> GLIVDTRDVEERVHVMRETKLAPTVAHGVFNPEFGPAALSNKDPRLNEGVVLDEVIFSKHKGDTKMSAEDKALFRRCAADYASRLHSVLGTANAPLSIYEAIKGVDGLDAMEPDTAPGLPWALQGKRRGALIDFENGTVGPEVEAALKLMEKREYKFACQTFLKDEIRPMEKVRAGKTRIVDVLPVEHILYTRMMIGRFCAQMHSNNGPQIGSAVGCNPDVDWQRFGTHFAQYRNVWDVDYSAFDANHCSDAMNIMFEEVFRTEFGFHPNAEWILKTLVNTEHAYENKRITVEGGMPSGCSATSIINTILNNIYVLYALRRHYEGVELDTYTMISYGDDIVVASDYDLDFEALKPHFKSLGQTITPADKSDKGFVLGHSITDVTFLKRHFHMDYGTGFYKPVMASKTLEAILS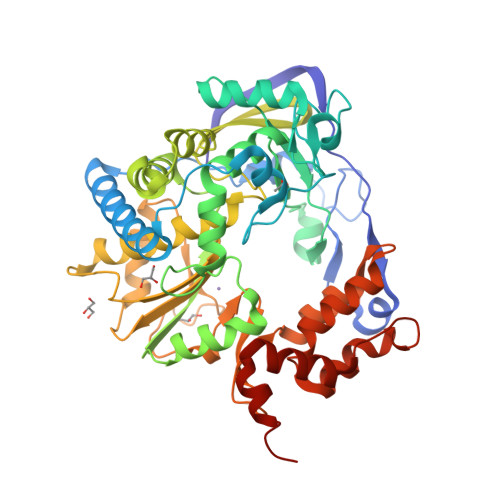FARRGTIQEKLISVAGLAVHSGPDEYRRLFEPFQGLFEIPSYRSLYLRWVNAVCGDAAALEHHHHHHH The intracellular Asp f3 is an abundant protein in A. fumigatus. It contains 168 amino acid residues and BLAST searches reveal considerable sequence homology to the thioredoxin superfamily, the peroxiredoxin (Prx) family, and the PRX5-like subfamily. We experimentally confirm the predicted peroxiredoxin activity of Asp f3 and demonstrate the functional contribution of its cysteine residues for catalytic activity. Finally, we provide evidence for the critical role of Asp f3 in fungal virulence, wherein it protects A. fumigatus against oxidative stress in vitro, and in vivo, in a murine model of invasive pulmonary aspergillosis.

Aspf3 wild type (WT) and its C31S/C61S variant crystallized as a homodimer and showed a typical thioredoxin-like fold. In the WT structure, both C31 and C61 reside in flexible loop regions (large B-factors and lack of well-defined electron density for one of the chains). The serine variant showed little overall structural change (RMSD 1.7 Å), with large deviation of the aforementioned loops (residues 24–35 and 58–64 RMSD > 4.0 Å). Disruption of the intermolecular disulfide bond in C31S/C61S variant extends the α-helix by 6 residues resulting in a significant movement of S61 by ~7–9 Å from the position occupied by C61 in the WT structure, analogous to the movement of C62 in the reduced form of Ahp115. A corresponding movement of S31 by 4–5 Å is likely driven by formation of a hydrogen bond to backbone oxygen of F57. The dimer interface comprises an area of ~710 Å2 and ~730 Å2 for WT and C31S/C61S variant, respectively. The slight increase in the overall dimer interface area for C31S/C61S (~730 Å2) is due to the fact that the loop connecting residues 24–31 is ordered in both protomers, whereas the backbone cannot be traced in one of the protomers in the WT structure. The WT, as well as C31S/C61S variant, exhibited close similarity to oxidized and reduced forms of Ahp1, respectively. S61 in C31S/C61S of Asp f3 becomes more buried, much like C62 in the reduced form of Ahp1. Therefore, we expect that the structure of the C31S/C61S mutant to bear close resemblance with that of the reduced dimeric Asp f3 WT. A three-fold reduction of the WT catalytic efficiency rate (kcat/Km) was determined for C31A/C61A, and a ten-fold reduction for C31S/C61S with t-bOOH or H2O2, respectively.

>[2x]MGSGLKAGDSFPSDVVFSYIPWSEDKGEITASGIPINYNASKEWADKKVILFALPGAFTPVSSARHVPEYIEKLPEIRAKGVDVVAVLAYNDAYVMSAWGKANQVTGDDILFLSDPDARFSKSIGWADEEGRTKRYALVIDHGKITYAALEPAKNHLEFSSAETVLKHLHHHHHH Mutations in leucine-rich repeat kinase 2 (LRRK2), a multi-domain protein containing both a kinase and a GTPase, are a leading cause of the familial form of PD. LRRK2 is a 2527-residue, 286 kDa protein. Its N-terminal half is composed of armadillo (ARM), ankyrin (ANK) and leucine-rich repeat (LRR) domains. The C-terminal half contains a Ras-like guanosine triphosphatase (GTPase, or Ras of complex, ROC) domain, followed by a “C-terminal of ROC” (COR) domain, a kinase domain and a WD40 domain, with the latter found at the C terminus.

In this study, we present cryo-ET structures of full-length LRRK2 bound to microtubules in the inactive, autoinhibited conformation. From dataset (2) (LRRK2I2020T with MLi-2 on pre-formed microtubules), we performed focused refinement from the map including both the microtubule and LRRK2 and obtained a 7.8 Å map of LRRK2 only, which showed the highest LRRK2 resolution after subtomogram analysis. Our model of full-length LRRK2 on microtubules is similar to the published cryo-EM models of in-solution, autoinhibited full-length LRRK212–14, with the LRR domain blocking the kinase’s active site. As was the case with the structures of in-solution LRRK2, the ARM domain is flexible in our map. In agreement with those structures and the proposal that the N-terminal repeats constrain conformational changes in LRRK2, the kinase in our full-length LRRK2 adopted an inactive, open conformation in the presence of the type-I inhibitor MLi-2. Similar to the structure of LRRK2RCKW on microtubules, our model showed two pseudo two-fold symmetry axes, one centered at the COR:COR interface between two LRRK2s in a dimer, and a WD40:WD40 interface between neighboring dimers. We resolved these clashes by shifting the N-terminal ARM/ANK domains of each LRRK2 away from its own WD40 domain. This suggests that a novel WD40:ARM interaction is involved in stabilizing the oligomerization of autoinhibited full-length LRRK2 on microtubules. The distribution of these angles in our samples peaked at around 90° (θ angle), leading to ring-like structures around the microtubule, in contrast to the right-handed helices with helical angles around 33° observed with the active-like forms of LRRK219,22. Instead, the most frequently observed species were individual dimers and short oligomers consisting of 2–6 LRRK2 dimers. In contrast, our in vitro reconstituted microtubule-bound filaments of autoinhibited LRRK2 revealed a stabilized N-terminal half (ARM/ANK/LRR domains) covering the kinase’s active site.

> HKLVLAALNRFIGNPGIQKCGLKVISSIVHFPDALEMLSLEGAMDSVLHTLQMYPDDQEIQCLGLSLIGYLITKKNVFIGTGHLLAKILVSSLYRFKDVAEIQTKGFQTILAILKLSASFSKLLVHHSFDLVIFHQMSSNIMEQKDQQFLNLCCKCFAKVAMDDYLKNVMLERACDQNNSIMVECLLLLGADANQAKEGSSLICQVCEKESSPKLVELLLNSGSREQDVRKALTISIGKGDSQIISLLLRRLALDVANNSICLGGFCIGKVEPSWLGPLFPDKTSNLRKQTNIASTLARMVIRYQMKSAVEEGTASGSDGNFSEDVLSKFDEWTFIPDSSMDSVFAQSDDLDSEGSEGSFLVKKKSNSISVGEFYRDAVLQRCSPNLQRHSNSLGPIFDHEDLLKRKRKILSSDDSLRSSKLQSHMRHSDSISSLASEREYITSLDLSANELRDIDALSQKCCISVHLEHLEKLELHQNALTSFPQQLCETLKSLTHLDLHSNKFTSFPSYLLKMSCIANLDVSRNDIGPSVVLDPTVKCPTLKQFNLSYNQLSFVPENLTDVVEKLEQLILEGNKISGICSPLRLKELKILNLSKNHISSLSENFLEACPKVESFSARMNFLAAMPFLPPSMTILKLSQNKFSCIPEAILNLPHLRSLDMSSNDIQYLPGPAHWKSLNLRELLFSHNQISILDLSEKAYLWSRVEKLHLSHNKLKEIPPEIGCLENLTSLDVSYNLELRSFPNEMGKLSKIWDLPLDELHLNFDFKHIGCKAKDIIRFLQQRLKKAVPYNRMKLMIVGNTGSGKTTLLQQLMKTKKSDLGMQSATVGIDVKDWPIQIRDKRKRDLVLNVWDFAGREEFYSTHPHFMTQRALYLAVYDLSKGQAEVDAMKPWLFNIKARASSSPVILVGTHLDVSDEKQRKACMSKITKELLNKRGFPAIRDYHFVNATEESDALAKLRKTIINESLNFKIRDQLVVGQLIPDCYVELEKIILSERKNVPIEFPVIDRKRLLQLVRENQLQLDENELPHAVHFLNESGVLLHFQDPALQLSDLYFVEPKWLCKIMAQILTVKVEGCPKHPKGIISRRDVEKFLSKKRKFPKNYMSQYFKLLEKFQIALPIGEEYLLVPSSLSDHRPVIELPHCENSEIIIRLYEMPYFPMGFWSRLINRLLEISPYMLSGRERALRPNRMYWRQGIYLNWSPEAYCLVGSEVLDNHPESFLKITVPSCRKGCILLGQVVDHIDSLMEEWFPGLLEIDICGEGETLLKKWALYSFNDGEEHQKILLDDLMKKAEEGDLLVNPDQPRLTIPISQIAPDLILADLPRNIMLNNDELEFEQAPEFLLGDGSFGSVYRAAYEGEEVAVKIFNKHTSLRLLRQELVVLCHLHHPSLISLLAAGIRPRMLVMELASKGSLDRLLQQDKASLTRTLQHRIALHVADGLRYLHSAMIIYRDLKPHNVLLFTLYPNAAIIAKIADYGTAQYCCRMGIKTSEGTPGFRAPEVARGNVIYNQQADVYSFGLLLYDILTTGGRIVEGLKFPNEFDELEIQGKLPDPVKEYGCAPWPMVEKLIKQCLKENPQERPTSAQVFDILNSAELVCLTRRILLPKNVIVECMVATHHNSRNASIWLGCGHTDRGQLSFLDLNTEGYTSEEVADSRILCLALVHLPVEKESWIVSGTQSGTLLVINTEDGKKRHTLEKMTDSVTCLYCNSFSKQSKQKNFLLVGTADGKLAIFEDKTVKLKGAAPLKILNIGNVSTPLMCLSESTNSTERNVMWGGCGTKIFSFSNDFTIQKLIETRTSQLFSYAAFSDSNIITVVVDTALYIAKQNSPVVEVWDKKTEKLCGLIDCVHFLREVMVKENKESKHKMSYSGRVKTLCLQKNTALWIGTGGGHILLLDLSTRRLIRVIYNFCNSVRVMMTAQLGSLKNVMLVLGYNRKNTEGTQKQKEIQSCLTVWDINLPHEVQNLEKHIEVRKELAEKMRRTSVE>[2x]MLSNLKTGNNILGLPEFELNGCRFLYKKGIEKTIITFSAFPPKDIAQKYNYIKDFLSSNYTFLAFLDTKYPEDDARGTYYITNELDNGYLQTIHCIIQLLSNTNQEDTY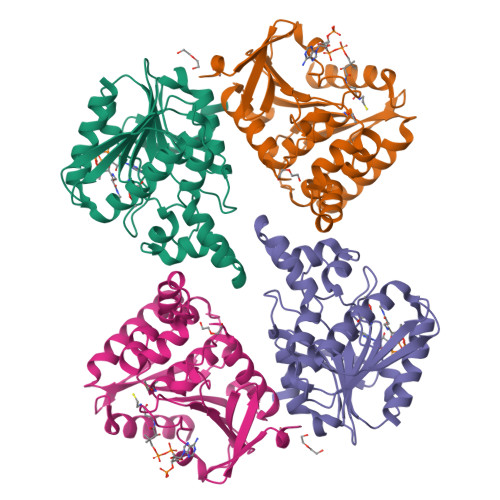LLGSSKGGVGALLLGLTYNYPNIIINAPQAKLADYIKTRSKTILSYMLGTSKRFQDINYDYINDFLLSKIKTCDSSLKWNIHITCGKDDSYHLNELEILKNEFNIKAITIKTKLISGGADNEAIAHYREYFKTIIQNILEHHHHHH>MAAPARDPPGYRYAAAILPTGSILSTIEVASHRRLFDFFAAVRSDENSLYDVEFDALLGSYCNTLSLVRFLELGLSVACVCTKFPELAYMNEGRVQFEVHQPLIARDGPHPVEQPVHNYMTKVIDRRALNAAFSLATEAIALLTGEALDGTGISLHRQLRAIQQLARNVQAVLGAFERGTADQMLHVLLEKAPPLALLLPMQRYLDNGRLATRVARATLVAELKRSFCDTSFFLGKAGHRREAIEAWLVDLTTATQPSVAVPRLTHADTRGRPVDGVLVTTAAIKQRLLQSFLKVEDTEADVPVTYGEMVLNGANLVTALVMGKAVRSLDDVGRHLLDMQEEQLEANRETLDELE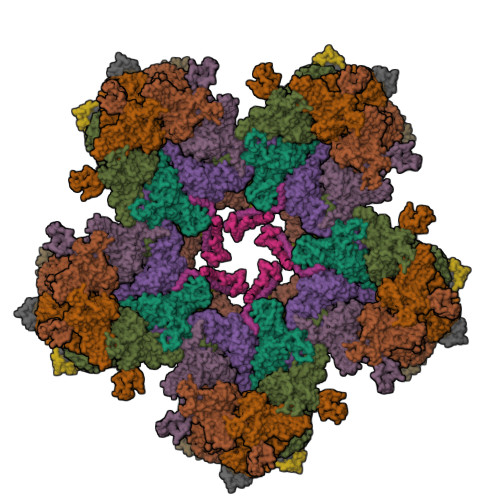SAPQTTRVRADLVAIGDRLVFLEALERRIYAATNVPYPLVGAMDLTFVLPLGLFNPAMERFAAHAGDLVPAPGHPEPRAFPPRQLFFWGKDHQVLRLSMENAVGTVCHPSLMNIDAAVGGVNHDPVEAANPYGAYVAAPAGPGADMQQRFLNAWRQRLAHGRVRWVAECQMTAEQFMQPDNANLALELHPAFDFFAGVADVELPGGEVPPAGPGAIQATWRVVNGNLPLALCPVAFRDARGLELGVGRHAMAPATIAAVRGAFEDRSYPAVFYLLQAAIHGNEHVFCALARLVTQCITSYWNNTRCAAFVNDYSLVSYIVTYLGGDLPEECMAVYRDLVAHVEALAQLVDDFTLPGPELGGQAQAELNHLMRDPALLPPLVWDCDGLMRHAALDRHRDCRIDAGGHEPVYAAACNVATADFNRNDGRLLHNTQARAADAADDRPHRPADWTVHHKIYYYVLVPAFSRGRCCTAGVRFDRVYATLQNMVVPEIAPGEECPSDPVTDPAHPLHPANLVANTVKRMFHNGRVVVDGPAMLTLQVLAHNMAERTTALLCSAAPDAGANTASTANMRIFDGALHAGVLLMAPQHLDHTIQNGEYFYVLPVHALFAGADHVANAPNFPPALRDLARDVPLVPPALGANYFSSIRQPVVQHARESAAGENALTYALMAGYFKMSPVALYHQLKTGLHPGFGFTVVRQDRFVTENVLFSERASEAYFLGQLQVARHETGGGVNFTLTQPRGNVDLGVGYTAVAATGTVRNPVTDMGNLPQNFYLGRGAPPLLDNAAAVYLRNAVVAGNRLGPAQPLPVFGCAQVPRRAGMDHGQDAVCEFIATPVATDINYFRRPCNPRGRAAGGVYAGDKEGDVIALMYDHGQSDPARPFAATANPWASQRFSYGDLLYNGAYHLNGASPVLSPCFKFFTAADITAKHRCLERLIVETGSAVSTATAASDVQFKRPPGCRELVEDPCGLFQEAYPITCASDPALLRSARDGEAHARETHFTQYLIYDASPLKGLSL[6x];>MITDCFEADIAIPSGISRPDAAALQRCEGRVVFLPTIRRQLALADVAHESFVSGGVSPDTLGLLLAYRRRFPAVITRVLPTRIVACPVDLGLTHAGTVNLRNTSPVDLCNGDPVSLVPPVFEGQATDVRLESLDLTLRFPVPLPTPLAREIVARLVARGIRDLNPDPRTPGELPDLNVLYYNGARLSLVADVQQLASVNTELRSLVLNMVYSITEGTTLILTLIPRLLALSAQDGYVNALLQMQSVTREAAQLIHPEAPMLMQDGERRLPLYEALVAWLAHAGQLGDILALAPAVRVCTFDGAAVVQSGDMAPVIRYP[2x];> MKTKPLPTAPMAWAESAVETTTSPRELAGHAPLRRVLRPPIARRDGPVLLGDRAPRRTASTMWLLGIDPAESSPGTRATRDDTEQAVDKILRGARRAGGLTVPGAPRYHLTRQVTLTDLCQPNAERAGALLLALRHPTDLPHLARHRAPPGRQTERLAEAWGQLLEASALGSGRAESGCARAGLVSFNFLVAACAAAYDARDAAEAVRAHITTNYGGTRAGARLDRFSECLRAMVHTHVFPHEVMRFFGGLVSWVTQDELASVTAVCSGPQEATHTGHPGRPRSAVTIPACAFVDLDAELCLGGPGAAFLYLVFTYRQCRDQELCCVYVVKSQLPPRGLEAALERLFGRLRITNTIHGAEDMTPPPPNRNVDFPLAVLAASSQSPRCSASQVTNPQFVDRLYRWQPDLRGRPTARTCTYAAFAELGVMPDDSPRCLHRTERFGAVGVPVVILEGVVWRPGGWRACA;>[6x]MAAPQFHRPSTITADNVRALGMRGLVLATNNAQFIMDNSYPHPHGTQGAVREFLRGQAAALTDLGVTHANNTFAPQPMFAGDAAAEWLRPSFGLKRTYSPFVVRDPKTPSTP> AQPDIKFASKEYGVTIGESRIIYPLDAAGVMVSVKNTQDYPVLIQSRIYDENKEKESEDPFVVTPPLFRLDAKQQNSLRIAQAGGVFPRDKESLKWLCVKGIPPKDEDIWVDDATNKQKFNPDKDVGVFVQFAINNCI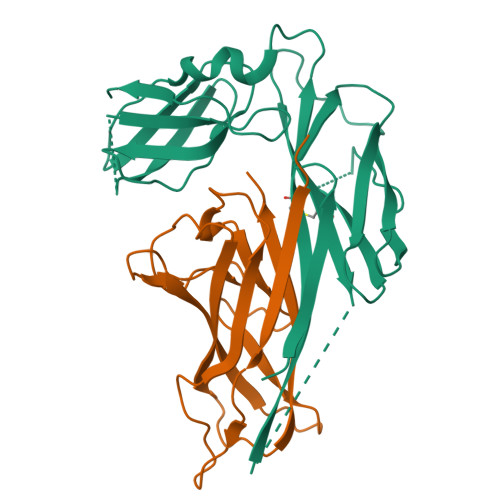KLLVRPNELKGTPIQFAENLSWKVDGGKLIAENPSPFYMNIGELTFGGKSIPSHYIPPKSTWAFDLPKGLAGARNVSWRIINDQGGLDRLYSKNVTL;> ADLTSHHHHHHVEPARITLTYKEGAPITIMDNGNIDTELLVGTLTLGGYKTGTTSTSVNFTDAAGDPMYLTFTSQDGNNHQFTTKVIGKDSRDFDISPKVNGENLVGDDVVLATGSQDFFVRSIGSKGGKLAAGKYTDAVTVTVSNQ> MEEHTEAGSAPEMGAQKALIDNPADILVIAAYFLLVIGVGLWSMCRTNRGTVGGYFLAGRSMVWWPVGASLFASNIGSGHFVGLAGTGAASGLAVAGFEWNALFVVLLLGWLFAPVYLTAGVITMPQYLRKRFGGRRIRLYLSVLSLFLYIFTKISVDMFSGAVFIQQALGWNIYASVIALLGITMIYTVT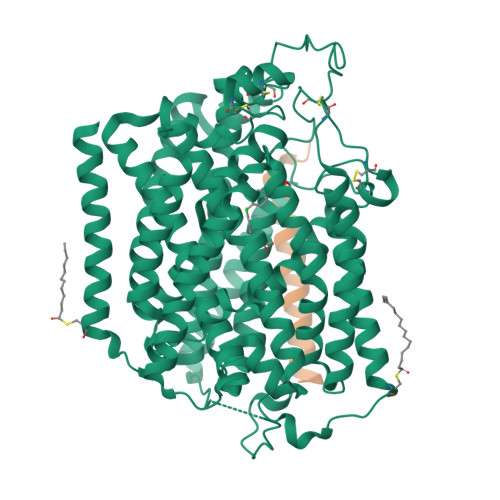GGLAALMYTDTVQTFVILGGACILMGYAFHEVGGYSGLFDKYLGAATSLTVSEDPAVGNISSFCYRPRPDSYHLLRHPVTGDLPWPALLLGLTIVSGWYWCSDQVIVQRCLAGKSLTHIKAGCILCGYLKLTPMFLMVMPGMISRILYPDEVACVVPEVCRRVCGTEVGCSNIAYPRLVVKLMPNGLRGLMLAVMLAALMSSLASIFNSSSTLFTMDIYTRLRPRAGDRELLLVGRLWVVFIVVVSVAWLPVVQAAQGGQLFDYIQAVSSYLAPPVSAVFVLALFVPRVNEQGAFWGLIGGLLMGLARLIPEFSFGSGSCVQPSACPAFLCGVHYLYFAIVLFFCSGLLTLTVSLCTAPIPRKHLHRLVFSLRHSKEEREDLDADEQQGSSLPVQNGCPESAMEMNEPQAPAPSLFRQCLLWFCGMSRGGVGSPPPLTQEEAAAAARRLEDISEDPSWARVVNLNALLMMAVAVFLWGFYA;> MSALSLLILGLLTAVPPASCQQGLGNLQPWMQGLIAVAVFLVLVAIAFAVNHFWCQ>GRKERERLEEKLEDANERIAELVKLEERQRIARDLEDTLGQKLSLIGLKSDLARKLIYKDPEQAARELKSVQQTARTSLNEVRKIVSSMKGIRLKDELINIKQILEAADIMFIYEEEKWPENISLLNENILSMCLKEAVTNVVKHSQAKTCRVDIQQLWKEVVITVSDDGTFKGEENSFSKGHGLLGMRERLEFANGSLHIDTENGT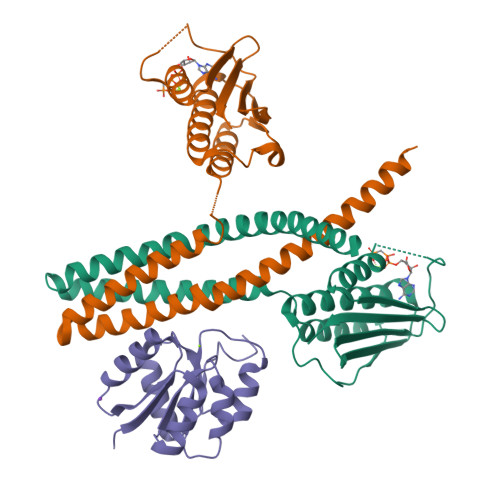KLTMAIPNNSK[4x];>GSGSMISIFIAEDQQMLLGALGSLLNLEDDMEVVGKGTTGQDAVDFVKKRQPDVCIMDIEMPGKTGLEAAEELKDTGCKIIILTTFARPGYFQRAIKAGVKGYLLKDSPSEELANAIRSVMNGKRIYAPELMEDLYSEA[2x]>[4x]MAKPQV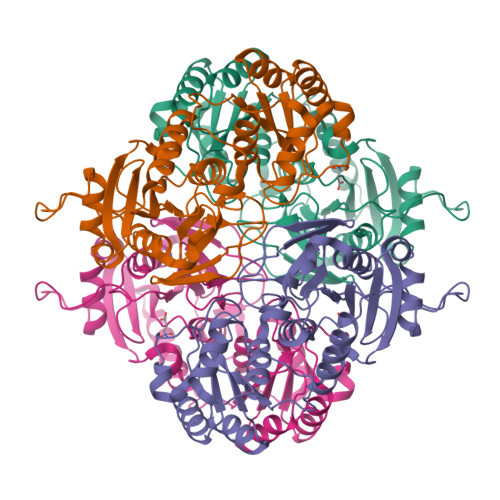TILATGGTIAGSGESSVKSSYSAGAVTVDKLLAAVPAINDLATIKGEQISSIGSQEMTGKVWLKLAKRVNELLAQKETEAVIITHGTDTMEETAFFLNLTVKSQKPVVLVGAMRSGSSMSADGPMNLYNAVNVAINKASTNKGVVIVMNDEIHAAREATKLNTTAVNAFASPNTGKIGTVYYGKVEYFTQSVRPHTLASEFDISKIEELPRVDILYAHPDDTDVLVNAALQAGAKGIIHAGMGNGNPFPLTQNALEKAAKSGVVVARSSRVGSGSTTQEAEVDDKKLGFVATESLNPQKARVLLMLALTKTSDREAIQKIFSTY>MAPTSSSTKKTQLQLEHLLLDLQMILNMLNNYDNPKLTRMLTFKFYMPKKATELKHLQCLEEELKPLEEALNQAQSKNFHLDPRDLISNINVIVLELKGSETTFMCEYA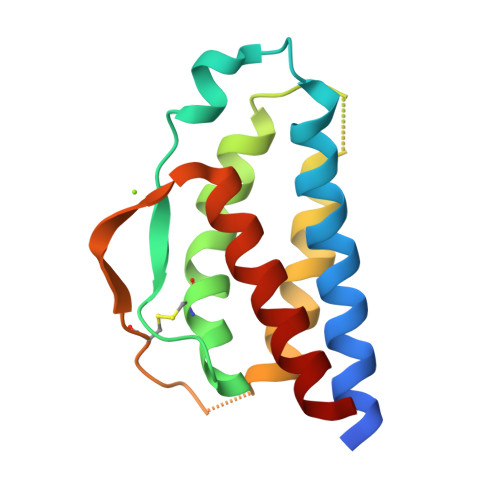DETATIIEFLNRWITFCQSIISTLT[4x]>[2x]GPGMAVKHLIVLKFKDEITEAQKEEFFKTWVNLVNIIPAMKDVYWGKDVTQK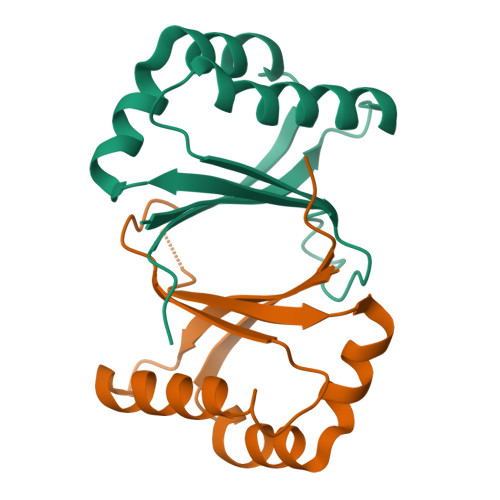NKEEGYTHIVEVTFESVETIQDYIIHPAHVGFGDVYRSFWEKLLIFDYTPRK8-bromo-4H-[1,2,4]oxadiazolo[3,4-c][1,4]benzoxazin-1-one 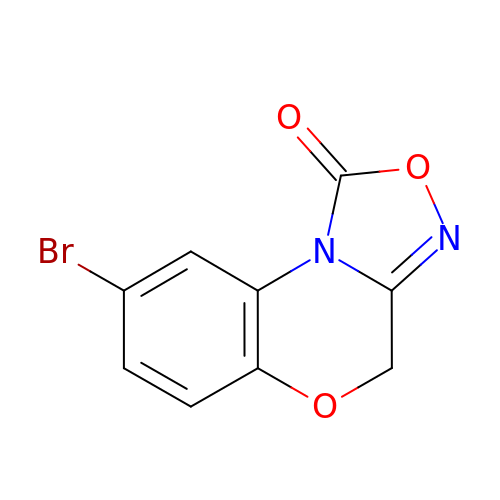| C9 H5 Br N2 O3 | MUDRLQRJCGJJTB-UHFFFAOYSA-N4-azaniumylbutylazanium | C4 H14 N2 | 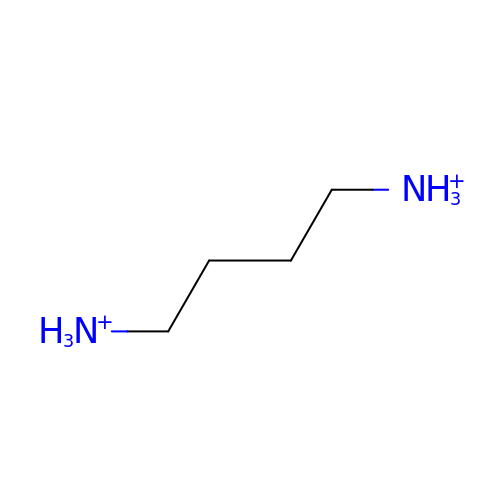KIDHWZJUCRJVML-UHFFFAOYSA-P>GASGSGTGSGSMSTLYLTQPDAVLSKKHEAFHVALKQEDGSWKKQPIPAQTLEDIVLLGYPSITGEALGYALELGLPVHYLTQFGKYVGSALPSESRNGQLRLAQFRAHEDPIQRLDIVKAFVKGKVHNQYNLLYRRGQVDNPLKGRGKLVMRQQTLEQVRGIEGLAAREYFASWQEMLGHEWTFTGRFRRPPTDPVNALLSFGYGLLRTQVTAAVHIAGLDPYIGFLHETTRGQPAMILDLMEEFRALVADSVVLTVLKQREIQRQDFTESLGAFRLTDSATKTFLGAFDRKLSSEFKHPIFNYKCT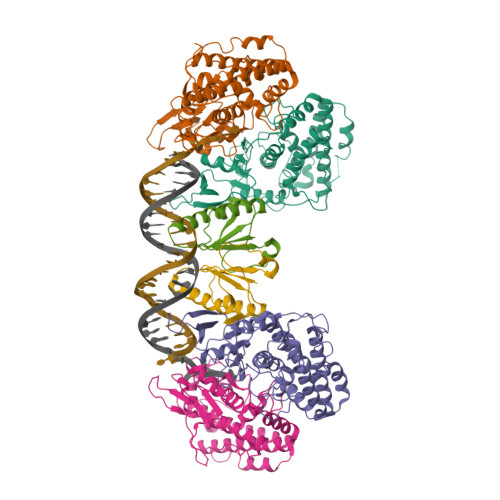YRRAIELQARLLARHLQEGVVYEPLVIR[4x];>[2x]GASGSGTGSGSMLYLIIYDVPATKAGNKRRTRLFDLLSGYGKWRQFSVFECFLSVKQFAKLQTAMEKLIKLDEDAVCIYVLDENTVQRTITYGTPQPEKPGSIII>XELENIVANTVLLKAREGGGGNRKGKSKKWRQMLQFPHISQCEELRLSLERDYHSLCERQPIGRLLFREFCATRPELSRCVAFLDGVAEYEVTPDDKRKACGRQLTQNFLSHTGPDLIPEVPRQLVTNCTQRLEQGPCKDLFQELTRLTHEYLSVAPFADYLDSIYFNRFLQWKWLERQPVTKNTFRQYRVLGKGGFGEVCACQVRATGKMYACKKLEKKRIKKRKGEAMALNEKQILEKVNSRFVVSLAYAYETKDALCLVLTLMNGGDLKFHIYHMGQAGFPEARAVFYAAEICCGLEDLHRERIVYRDLKPENILLDDHGHIRISDLGLAVHVPEGQTIKGRVGTVGYMAPEVVKNERYTFSPDWWALGCLLYEMIAGQSPFQQRKKKIKREEVERLVKEVPEEYSERFSPQARSL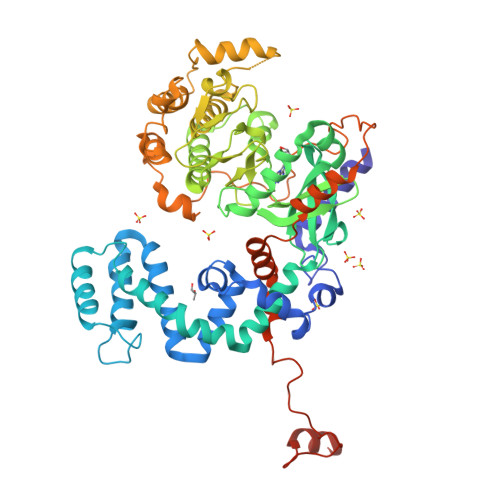CSQLLCKDPAERLGCRGGSAREVKEHPLFKKLNFKRLGAGMLEPPFKPDPQAIYCKDVLDIEQFSTVKGVELEPTDQDFYQKFATGSVPIPWQNEMVETECFQELNVFGLDGSVPPDLDWKGQPPAPPKKGLLQRLFSRQDCCGNCSDSEEELPTRL[2x]> MEVKELERDKNRVVLEYVFGAEEIAQAEDKAVRYLNQRVEIPGFRKGRIPKNVLKMKLGEEFQEYTLDFLMDLIPDTLKDRKLILSPIVTERELKDVTARVVVEVHEEPEVRIGDISKIEVEKVDEEKVLEKYVERRIEDLRESHALLEPKEGPAEAGDLVRVNMEVYNEEGKKLTSREYEYVISEDEDRPFVKDLVGKKKGDVVEIEREYEGKKYTYKLEVEEVYKRTLPEIGDELAKSVNNEFETLEQLKESLKKEGKEIYDVEMKESMREQLLEKLPEI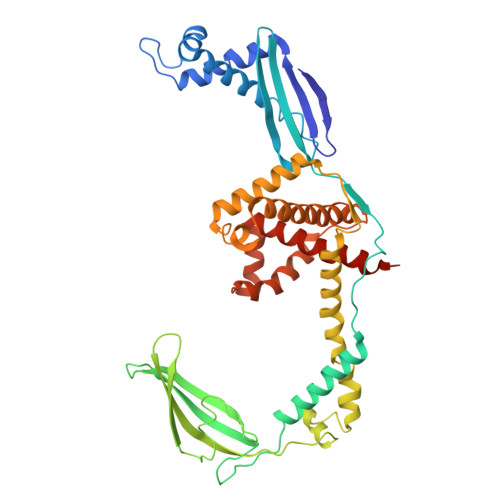VEIEISDRTLEILVNEAINRLKREGRYEQIVSSYESEEKFREELKERILDDIKRDRVIEVLAQEKGISVNDEELEKEAEELAPFWGISPDRAKSLVKARQDLREELRWAILKRKVLDLLLQEVEHHHHHH> MKKILIVDDEKPISDIIKFNMTKEGYEVVTAFNGREALEQF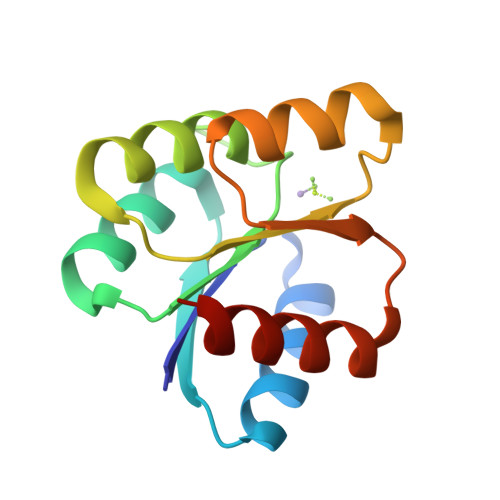EAEQPDIIILDLMLPEIDGLEVAKTIRKTSSVPILMLSAKDSEFDKVIGLELGADDYVTKPFSNRELQARVKALLRRSQ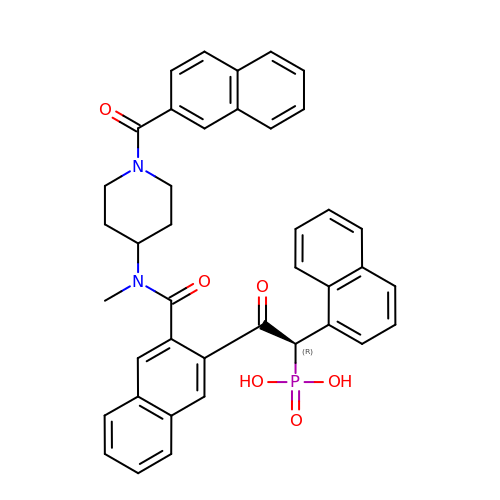2-[3-({METHYL[1-(2-NAPHTHOYL)PIPERIDIN-4-YL]AMINO}CARBONYL)-2-NAPHTHYL]-1-(1-NAPHTHYL)-2-OXOETHYLPHOSPHONIC ACID | C40 H35 N2 O6 P | XUJQPDQURBZEGJ-KXQOOQHDSA-N> GPLGSEQQPGDRCPRHVARIIAENDPPIRCDLTLQELLSEVQVDFEPSASEVVAMEGLMDEQHFIPHDPHSKKAAVQSLVIAIKTADLLLQMIHENVKRDIRTTCIQMANESYARADIVRDSLIAASQGKYTALGKIVFHSYTNFMPVNANESEKRAWMEMLGECTSHGNKLCEMANAQVEQETRDIINIMFKNIDDVVTQTTRAMRGVFDPPDTVKALSAAAQLIRVWEHDNVINDQSVSTSSVVTAALEANENLAKALRDVSGYAEVQFNRLCLSILTSAKERIDIIYHSARSQHLACNVRMNVAQQNLATFILTNARERPNDAVIRTRRAVANTGILLFTGQHIT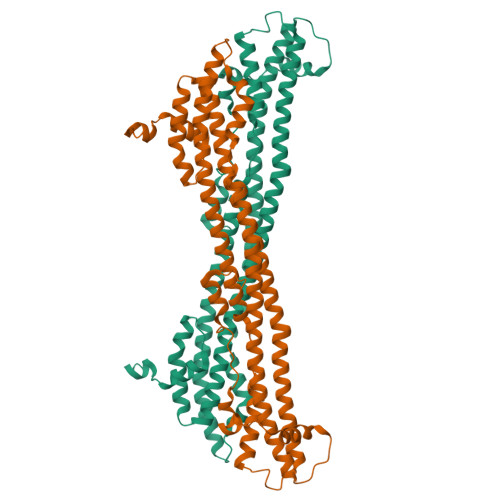RDALDKAAESKSVEEIVGMS>SRFADAVLDQYIGSIHSLCKDQHGCRFLQKQLDILGSKAADAIFEETKDYTVELMTDSFGNY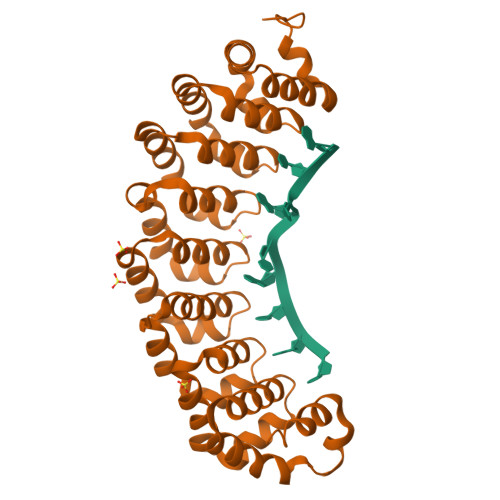LIQKLLEEVTTEQRIVLTKISSPHFVEISLNPHGTRALQKLIECIKTDEEAQIVVDSLRPYTVQLSKDLNGNHVIQKCLQRLKPENFQFIFDAISDSCIDIATHRHGCCVLQRCLDHGTTEQCDNLCDKLLALVDKLTLDPFGNYVVQYIITKEAEKNKYDYTHKIVHLLKPRAIELSIHKFGSNVIEKILKTAIVSEPMILEILNNGGETGIQSLLNDSYGNYVLQTALDISHKQNDYLYKRLSEIVAPLLVGPIRNTPHGKRIIGMLHLDS[2x]> MTYAVAFRLERGLVFAADTRTNAGVDNIAQYKKLQLWRQPGERVFVLLSAGNLAATQAVVSLINEHLSQETDDEVTTLFTAPNMYRAARVV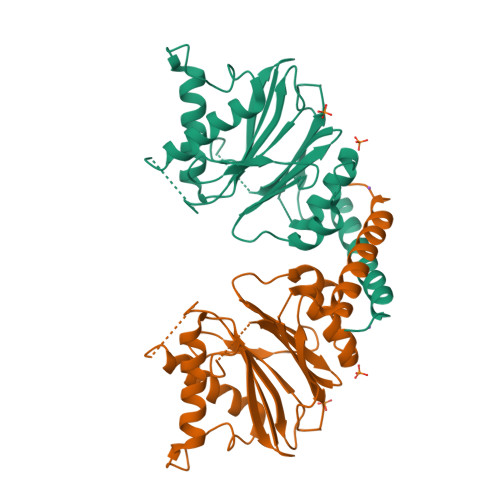GDAVREARSIDGAALEASKLGFNTNFIFGGQIKGERPRLFQIYPEGNFIEATDDTPFFQIGEHKYGKPILDRVARSDMRLGEAAKLMLLSFDSTLRSNLSVGMPIDLVIYERDTFDVTREKRISADDEYFRNLSNAWSDALRQAFSKIEEFDV> MRCIGISNRDFVEGVSGGSWVDIVLEHGSCVTTMAKNKPTLDFELIKTEAKQPATLRKYCIEAKLTNTTTDSRCPTQGEPSLNEEQDKRFVCKHSMVDRGWGNGCGLFGKGGIVTCAMFTCKKNMKGKVVQPENLEYTIVITPHSGEEHAVGNDTGKHGKEIKITPQSSITEAELTGYGTVTMECSPRTGLDFNEMVLLQMENKAWLVHRQWFLDLPLPWLPGADTQGSNWIQKETLVTFKNPHAKKQDVVVLGSQEGAMHTALTGATE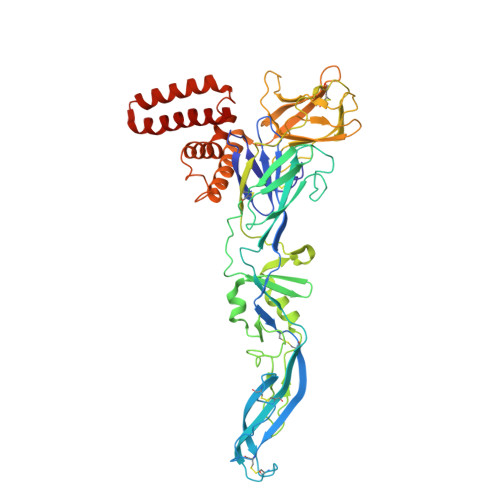IQMSSGNLLFTGHLKCRLRMDKLQLKGMSYSMCTGKFKVVKEIAETQHGTIVIRVQYEGDGSPCKIPFEIMDLEKRHVLGRLITVNPIVTEKDSPVNIEAEPPFGDSYIIIGVEPGQLKLNWFKKGSSIGQMIETTMRGAKRMAILGDTAWDFGSLGGVFTSIGKALHQVFGAIYGAAFSGVSWIMKILIGVIITWIGMNSRSTSLSVSLVLVGVVTLYLGVMVQA>MTCNFETADRRKRFWTTQVAACGQSSDDCGDCARPGLQLLCNGEGRITIATDNYVAGLALNILLTDASKADTGCGWTPGNRGGFWGDSFRSDNMRSGSKIRQVTARGSMRETVALIRAYAIDDLKKLVAYGVAKSVDVDLTYQGSNKIDMTIMIQGVDGNESRVGLTGERIANAWVWS[6x];>MAGPCYNPNEHYLPASFKGVPFDADSSDSEHGRNGAEAEFVFGERTGYADLGIKIRSYSIRARFQTNDHVALSNAFIAVLESTGPGLLVHPTRGPVMAACRSARVTDSKVDAAGVTYIDIDFVEANDTVTGFGLVGSLIALALSPIITATEESFKRYYSPENVRYYNSETVIATMAEAVQQVQTGYLALSGNDTSQEKWTIVRDFRNVLIDEFTFFDPANSWNVLRNGFSYLDSAAVGQDKFTILRNIINWSSSHSELDGESADAQNAIFSAVRVLATAYLSKAYMETVASTVNEGLAQYDQIAAILEQEAQIAQEDCHDNEFFLSIREFSVSVARVMVNRAYNSPALIVYSFPGTMHSLVVAWEIFGDAKRSRELEGRNTGAPWAIGPKVIAERVRA[6x];>[3x]MTTTKTFDERNRDTQDGFERHVFRKLDHTDTGAIVTVEGSGTMDEDVPVINSGYGFNPEDDEELEVFLLSDGSDASGKFGVMTIPRNKQRKWPKKTGGIQHPFNADKFVQLDDDSIWLKDGKFTLGDNRSLSITVEGNNVVIDTGGGELDIRSSKLMHNGVNIGDSHVHPQQADSDGDTEADTDPPKRD;>MIKPMRIFIGGEELETYTSARLQRTKKQLTGSLTVEIFLNYVPSKPVIVNAVRGKEILVYVMGELAFTGIIDKRKGKTVAGSQPRDASGRFAYSGGPGSMSDEGGSDVTVNFAKGQGYSVTLTARGRTKYLVDSSHSHPTGSFKDTSDRKVIEALVKEHKVVLDWQGTEVKEPKITLRDGNRIFNEIFERCNQNCHFAYETRDGKLLVTDGTTGVVGEDIVLGQNILDFSAEQSEDRANSEITVKGHRVAKDVWGKNAIVQPVQSVADSWVGANIPLTIQHYGDATN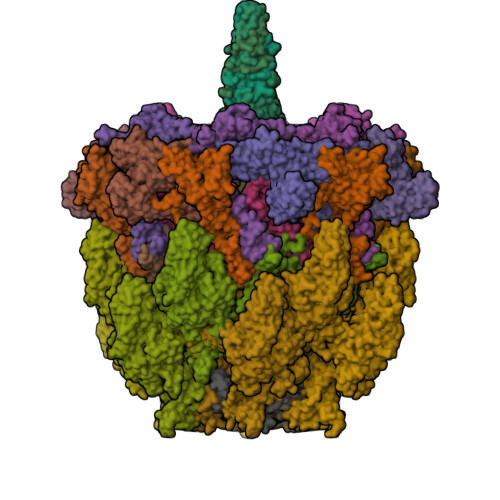ESLQRRAKFEADRRAAESKSVNVTVFHVAQQGGIPWDIGNIHYVEIPPEGIFDVMECVSLTYSVDAKSTLETQLELAPPPSESISGASSGLLSSISNSLADISTKGVARRVQAGIKLIAGQYPSTWTSAALSAITTPVNVIASVVNSLLLNEDESTPKQPPLRLPPE[3x];>MNVLVPGIDGMVSAGKFEYSGCCPPDFADMDECTLATSYVGLLPSGPLWDRAKYEAITTITATGNCAACWTEDHCPTLVDYAVNVGARLASVIDMTLWPAVRESDPFTAVTSTADWLERFKWVNCFETSCRSKALGEITPIEYMTECGPVYVAINYPPSIKQAFESALIKSLERLSMGIIKNLASINFVIEPLKVRVVPLDTTNACENETLCVTFEKTSDFFDGVNQNPCGIPSPVAAYIDRDVMQLPSELPKYIWPGHMAAECVVRSLLSHVSRFCVVRTDQTPD[6x];>MACTIQRPEPQALRDKIATRFSTNVLGGAEIIPESNEFYVVTLEYAMQEEFFAFAEQMWREQDPRYACCENLVKMAARRGVYPKPAQFAQGYVRMTGVPGSALNQNLRFQFENQTYEAASVVPDQLPATGVLVLRVSAVTPGPSGNIRVTEGSLVTPVPGISSAVTAYGGNFCGGDDAEECEPFRTRYLQRLQYEPRLTVEWLKSKAMEWPCVTDVFDLGPNCCSVNALGEVECPNNIEFYVLFRDTFDCGLAPQCVVDEITDWLFGSPQGLGQGEAEFGICGKVRTATAVNLDIYLNGLSCATPAQARVVEQRITDFINRHPPSTNLTVEQLRFIGLQVLGSSFAFDVAIRSPGDASQSGLRFNACGDAEIDCDYKACLNSVQVINNNVTTSGCL[12x];>[12x]MAQDALSDGFVRLCIDPSLNFFGEGCKILVEGQITDDATAAENVVTCVNSELDLVERFGQGSVLTESLRKVFCMCKSGVSVYALPRADAAAAVSAVYTLTVTGTALTDGRVQLYMGEAEYSLDIGVDEGDTPTQIAAKIVAAISPDFPYEATAAAGVITLTARNGGTIGNHLSVIYTNLGSCTSVTPEGVTVAFAQTTPGSVNPEPNDYASVVNECCFAVYVLSSDDTDWQENLRDWIRSAWDCSKPQCFGHGYVFNKGTLGQVLADGDNSAELSRLALPTTYPVLPYLTNAAYGALSACSTCENPELNVQGQTYGLLSCINMPESCTPGWEFTEVTQLQNNGFVVSGPATTSGQGNFTSPYIYNDVTNYLRDEKNRPNATFRDASSRRLAAATGVALATFLQQFNGLAVFTKNTNIKTGIIGTNLRLMLGKIRKWASDNVGVLFSEFDNINEDIQLVSDFDVQPKCVGQPGVFHLNMRYRPPVRGARINVNLVPALFDNCDR;>MACNKQNGVKNILITFTHCDTGEVIGPISHEQPDDTLPTYKTCAWTNTALTNGAVMRSASNATMTLPVVRDPRVPLAWYQGCAQIDAQVEKFDGTVMTLTEGAVTEPEESDGRAVTMTIIAAEIDELLPPGSLAAA[12x]> GSMAGWQSYVDNLMCDGCCQEAAIVGYCDAKYVWAATAGGVFQSITPAEIDVIIGKDREGFFTNGLTLGGKKCSV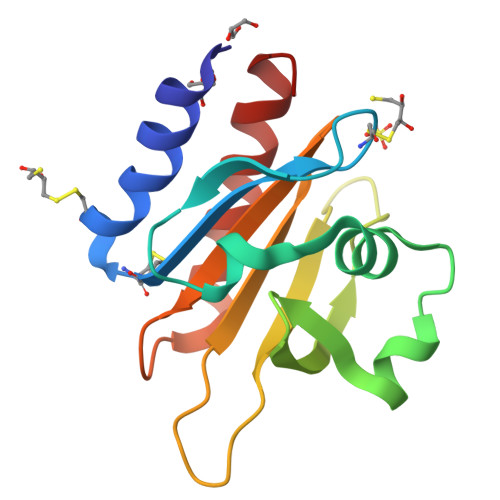IRDSLYVDSDCTMDIRTKSQGGEPTYNVAVGRAGRVLVFVMGKEGVHGGGLNKKAYSMAKYLRDSGF>MANVDEAILKRVKGWAPYVDAKLGFRNHWYPVMFSKEINEGEPKTLKLLGENLLVNRIDGKLYCLKDRCLHRGVQLSVKVECKTKSTITCWYHAWTYRWEDGVLCDILTNPTSAQIGRQKLKTYPVQEAKGCVFIYLGDGDPPPLARDTPPNFLDDDMEILGKNQIIKSNWRLAVENGFDPSHIYIHKDSILVKDNDLALPLGFAPGGDRKQQTRVVDDDVVGRKGVYDLIGEHGVPVFEGTIGGEVVREGAYGEKIVANDISIWLPGVLKVNPFPNPDMMQFEWYVPIDENTHYYFQTLGKPCANDEERKKYEQEFESKWKPMALEGFNNDDIWAREAMVDFYADDKGWVNEILFESDEAIVAWRKLASEHNQGIQTQAHVSGLEHHH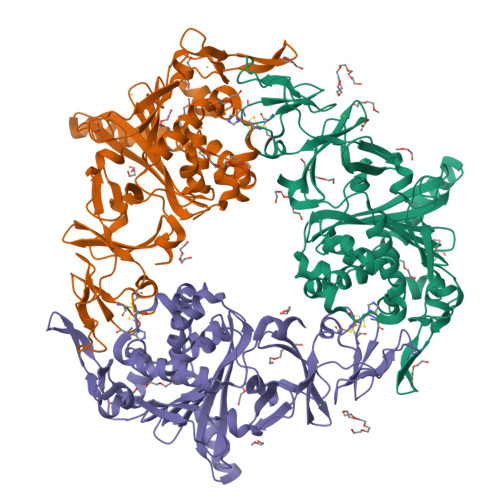HHH[3x]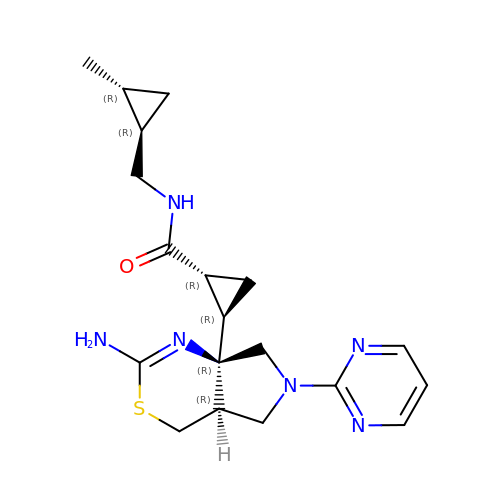(1R,2R)-2-[(4aR,7aR)-2-amino-6-(pyrimidin-2-yl)-4a,5,6,7-tetrahydropyrrolo[3,4-d][1,3]thiazin-7a(4H)-yl]-N-{[(1R,2R)-2-methylcyclopropyl]methyl}cyclopropane-1-carboxamide | C19 H26 N6 O S | UKXLLHCQBVONES-MPDRSUQMSA-N ETHYL (5S,8S,11R)-8-BENZYL-5-(3-TERT-BUTOXY-3-OXOPROPYL)-3,6,9-TRIOXO-11-{[(3S)-2-OXOPYRROLIDIN-3-YL]METHYL}-1-PHENYL-2-OXA-4,7,10-TRIAZATETRADECAN-14-OATE | C37 H50 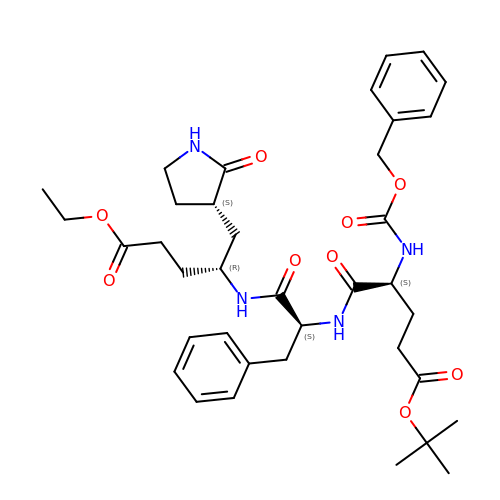N4 O9 | MMMLJIROCXIHMV-XJYHXZFBSA-N>[4x]SEFGCDGTLEQNDTTREVFLRFHNDVRKFIALGIYPNKVGVLGPAKNMYQLKWSCDLEEEAHESI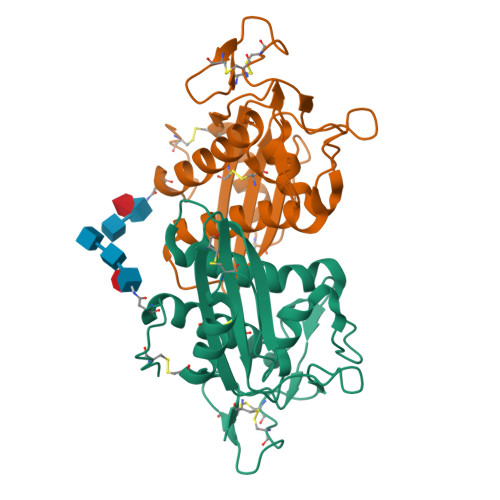YSCSYNPLLLHPQSYSKLLSVDLPDTDVVGATLEMWTEFMRIYGVNTKTNSYNPSFSQFANMAYSKNTKVGCSYKKCGGDTLVTCVYELGVKLPSHPQMWENGPTCVCVAYTDSICNDNNLCEYAPTSAR>TEDDDEDDYTEYKLTESIDNILVKMFKTNENNDKS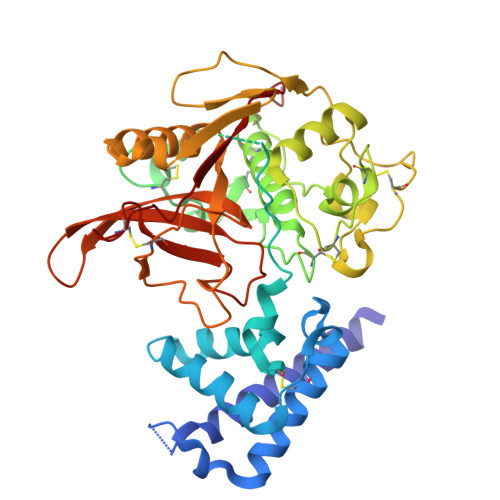ELIKLEEVDDSLKLELMNYCSLLKDVDTTGTLDNYGMGNEMDIFNNLKRLLIYHSEENINTLKNKFRNAAVCLKNVDDWIVNKRGLVLPELNYDLEYFNEHLYNDKNSPEDKDNKGKGVVHVDTTLEKEDTLSYDNSDNMFCNKEYCNRLKDENNCISNLQVEDQGNCDTSWIFASKYHLETIRCMKGYEPTKISALYVANCYKGEHKDRCDEGSSPMEFLQIIEDYGFLPAESNYPYNYVKVGEQCPKVEDHWMNLWDNGKILHNKNEPNSLDGKGYTAYESERFHDNMDAFVKIIKTEVMNKGSVIAYIKAENVMGYEFSGKKVQNLCGDDTADHAVNIVGYGNYVNSEGEKKSYWIVRNSWGPYWGDEGYFKVDMYGPTHCHFNFIHSVVIFNVDLPMNN[2x]> AAA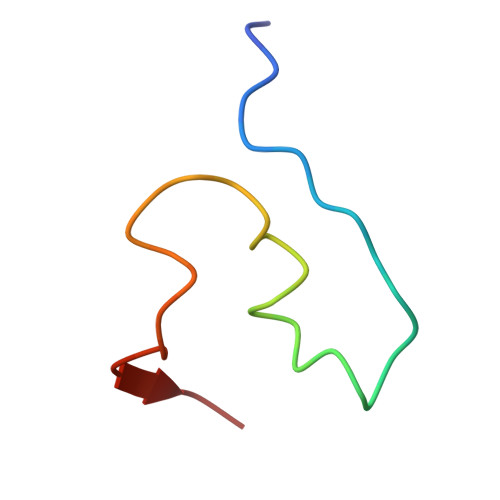AAAAAAAAAAAAAAAAAAAAAAAAAAAAAAAAAA>[4x]GSMVEPSLVLYGAPYERAVEV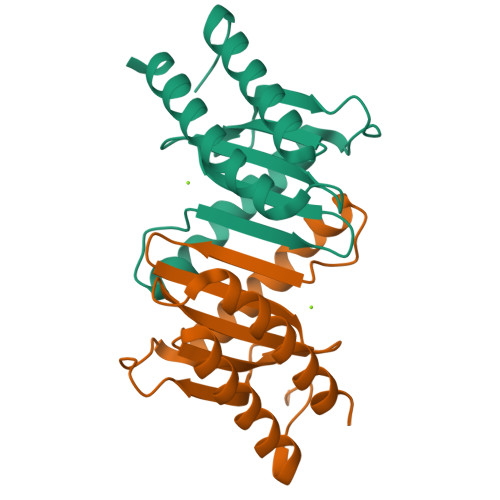LEETLRETGARYALLIDRKGFVLAHKEALWAPKPPPLDTLATLVASNAAATQALAKLLGEARFQEEVHQGERMGLYVDEAGEHALLVLVFDETAPLGKVKLHGKRAAEALARIAEEALANPPRLALDTEYREGAEALLDDLLRN> MAMKTQRKENVLFQNVK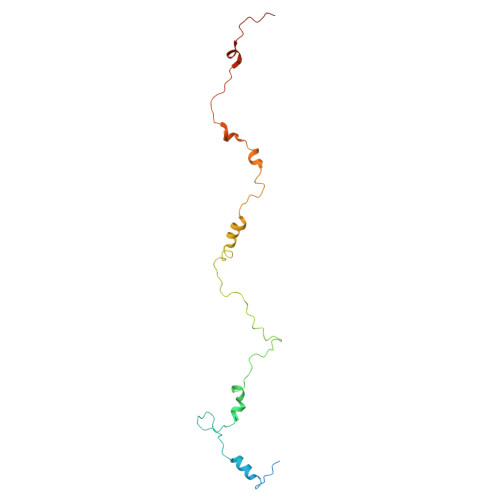PREIPLVDNPFSTYPYKHVITETQPTQAKNQAIWGLVQMGLSGEAAAMYGDVVVQKTTRACRKSEGGFKDVNTELWGTSPYLGRGDGEVYNMPASNQLLRGFESSLRGSRVRTQIDDKSFIPYTWQMIDVPLAAAKTSFIAGLDTRQQLAYGNP>[6x]MKDFLRLELPVLPLRNTVVLPHTTTGVDVGRLKSKRAVEEALSADRLLFLVTQKDPEVDDPAPEDLYAVGTLAVVKQAMRLPDGTLQVMVEARSRARLLSYVAAPYLRAVGEAIPEPPLKDPELARVLVNEVQEAFERYLQNHKTLRLDRYQQEAVKSTRDPAILADLVAHHATWTLEEKQTILETPEVEERLKRVLALLLRDLERFELDKKIAARVKEQMDQNQREYYLREQMKAIQKELGGGEDFLTEIEELRERIEKKGMPEPVKEKALKELKRLERMQPGSPEATVSRTYLDWLLEVPWTEADPEVLDISVTKRVLDEDHYGLKEVKERILEYLAVRQLTQGKEVKGHAPILCFVGPPGVGKTSLGKSIARSMNRRFHRISLGGVRDEAEIRGHRRTYIGALPGKIIQGMKQVGVVNPVFLLDEIDKLSSDWRGDPAAALLEVLDPEQNHTFTDHYLDVPYDLSKVFFITTANTLSTIPRPLLDRMEVIEIPGYTLHEKRAIARYFRWPFQVKEAGLEGRLEITDRAIERIVQEYTREAGVRNLDRELSKVARKAAKDYLEKPWEGVRVVDAEDLEAYLGVPKYRPDRAEKEPQVGAAQGLAWTPYGGTLLTIEAVAVPGTGKVNLTGNLGEVMKESAHAALTYLRAHREEWGLPEGFHKDYDLHIHVPEGATPKDGPSAGITIATALASALTGRPVRMDIAMTGEITLRGRVLPIGGVKEKLLAAHQAGIHRVILPKENAAELKEVPEEILKDLEIHFVEEVGEVLKLLLLPPPPPPAVQPDRPQPGVGA

In bacteria, Lon is a large hexameric ATP‐dependent protease that targets misfolded and also folded substrates, some of which are involved in cell division and survival of cellular stress. The N‐terminal domain of Lon facilitates substrate recognition, but how the domains confer such activity has remained unclear.

Here, we report the full‐length structure of Lon protease from Thermus thermophilus at 3.9 Å resolution in a substrate‐engaged state. The six N‐terminal domains are arranged in three pairs, stabilized by coiled‐coil segments and forming an additional channel for substrate sensing and entry into the AAA+ ring. Sequence conservation analysis and proteolysis assays confirm that this architecture is required for the degradation of both folded and unfolded substrates in bacteria.(2'S,3R,4'S,5'R)-6-chloro-4'-(3-chloro-2-fluorophenyl)-2'-(2,2-dimethylpropyl)-N-(trans-4-hydroxycyclohexyl)-2-oxo-1,2-dihydrospiro[indole-3,3'-pyrrolidine]-5'-carboxamide 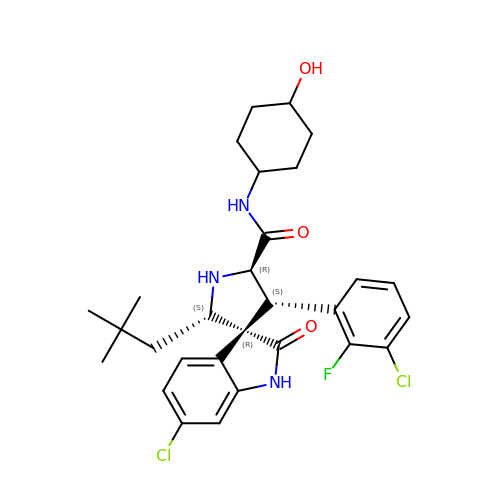| C29 H34 Cl2 F N3 O3 | IDKAKZRYYDCJDU-HBMMIIHUSA-N>GMTTPSHLSDRYELGEILGFGGMSEVHLARDLREHRDVAVKVLRADLARDPSFYLRFRREAQNAAALNHPAIVAVYDTGEAETPAGPLPYIVMEYVDGVTLRDIVHTEGPMTPKRAIEVIADACQALNFSHQNGIIHRDVKPANIMISATNAVKVMDFGIARAIADSGNSVTQTAAVIGTAQYLSPEQARGDSVDARSDVYSLGCVLYEVLTGEPPFTGDSPVSVAYQHVREDPIPPSARHEGLSADLDAVVLKALAKNPENRYQTAAEMRADLVRVHNG[2x];>GMTDMNPDIEKDQTSDEVTVETTSVFRADFLSELDAPAQAGTESAVSGVEGLPPGSALLVVKRGPNAGSRFLLDQAITSAGRHPDSDIFLDDVTVSRRHAEFRLENN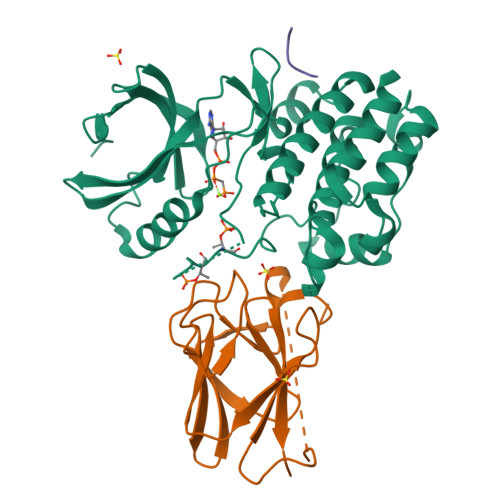EFNVVDVGSLNGTYVNREPVDSAVLANGDEVQIGKFRLVFLTGPKQGEDDGSTGGP[2x]>TFNLFVGDLNVNVDDETLRNAFKDFPSYLSGHVMWDMQTGSSRGYGFVSFTSQDDAQNAMDSMQGQDLNGRPLRINWA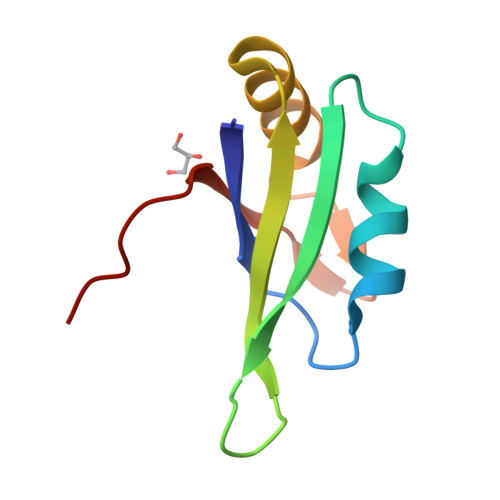AKLEH[2x]> TGEVKRPETSAPVPPLIKEATYIEATASGYMAEGVLNPTIILRRGQRVDMTLKNKLTEPTIVHWHGFDVNWHNDAHPSFAITPGESYNYSFDVVNRAGTYLYHPHPHGLTAKQFYMGQLGLVIVEDSGSDLGFKYGVNDLPLVISDRRFIGGAPVYNPTPMEMIAGFLGNAVLVNGVKDAVFKLSGGSYRLRLVNGSNARLYMLSIVKKNGDVVPMRLIAVDQGFLARPIEVRALFLAPAERAEVVVELGEGVYLLKNTPFDPMHLEMGHGMQEALPEGSEYTIATFLVEGKGEAVPVEALSDPPPEPPKPTRTRRFALSLSGMQWTINGMFWNASNPLFEHVSVEGVELWEIVNDKASMPHPMHLHGFPMWIIERKDSPRQVAELA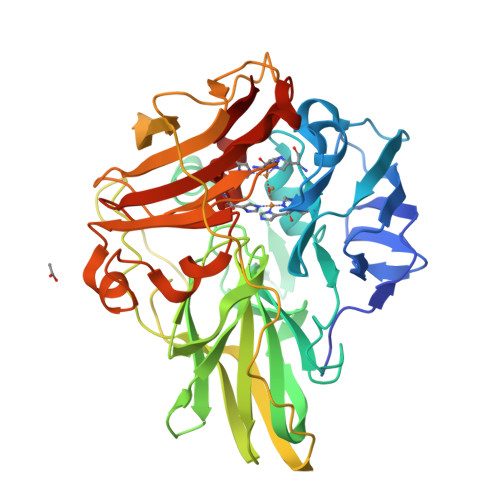VDNRGRLPTDLGLKDTVLIWPGETVKIVVNFDAKKRGQLFPFHCHNLEHEDGGMMINIAVK> GPGMSKEKILPLAARSKKAMLRQPKQVAYFSRDLNYKTHPDRSNLSYYYLPDGDIDNSIDLSVGSKHFLLGDSVEL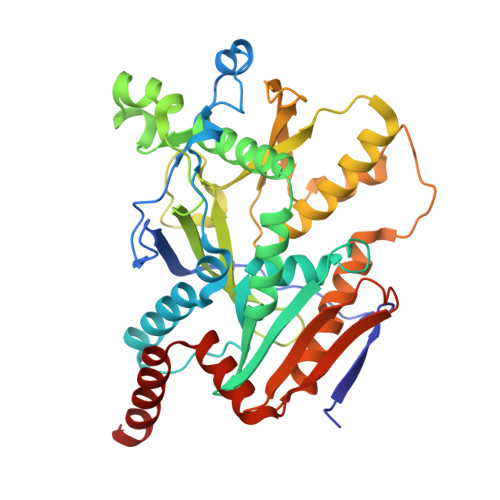SKLDPILLALKEIEKESGAKTKDRIITWRGIMRKLLTLPYDSEEDFVLDVVSFDGQLFIQFNVPYLKSKDVQKQGDTEFHKKLQFSGYKFEKMATLPKPWPECTRKEIDSRAKSKCNNIEQYGAIVRTGISRIKILIGGAVACTADYYDENDPLSRYIELKTTRTINQYKDMIAFEKKLFRTWAQCFLLGIPKIIYGFRDDNCILRTVEEFSTNDIPLMVKNNPLNEQPKKENCYMSSINFYGAVVEWLNESVKDDQVWKLSYAKRNRQYLVLKEVTDENEKQQIVDSAIPAWFKEWRSELRNSEGNI> GSRMSGNNMSTPLPAIVPAARKATAAVIFLHGLGDTGHGWAEAFAGIRSSHIKYICPHAPVRPVTLNMNVAMPSWFDIIGLSPDSQEDESG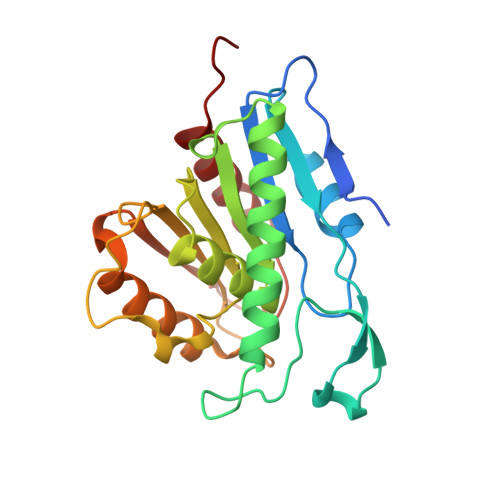IKQAAENIKALIDQEVKNGIPSNRIILGGFSQGGALSLYTALTTQQKLAGVTALSCWLPLRASFPQGPIGGANRDISILQCHGDCDPLVPLMFGSLTVEKLKTLVNPANVTFKTYEGMMHSSCQQEMMDVKQFIDKLLPPIDA> APFDDDDKIVGGYNCEENSVPYQVSLNSGYHFCGGSLINEQWVVSAGHCYKSRIQVRLGEHNIEVLEGNEQFINAAKIIRHPQYDRKTLNNDIMLIKLSSRAVINARV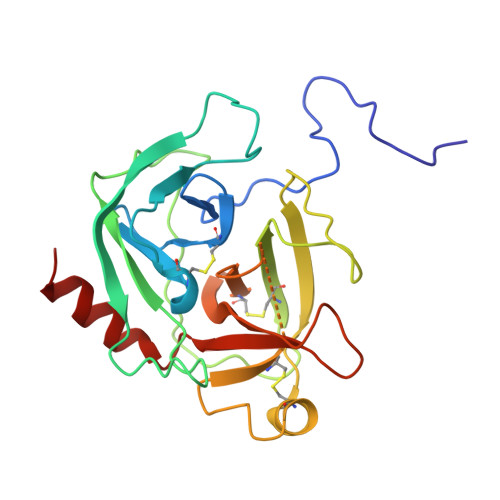STISLPTAPPATGTKCLISGWGNTASSGADYPDELQCLDAPVLSQAKCEASYPGKITSNMFCVGFLEGGKDSCQGDSGGPVVCNGQLQGVVSWGDGCAQKNKPGVYTKVYNYVKWIKNTIAANS> TEKFDFGTMVQWAYDHKYAEESKIAYEYALAAGSDSNARAFLATNSQAKHVKDCATMVRHYLRAETQALSMPAYIKARCKLATGEGSWKSILTFFNYQNIELITFINALKLWLKGIPKKNCLAFIGPPNTGKSMLCNSLIHFLGGSVLSFANHKSHFWLASLADTRAALVDDATHACWRYFDTYLRNALDGYPVSIDRKHKAAVQIKAPPLLVTSNID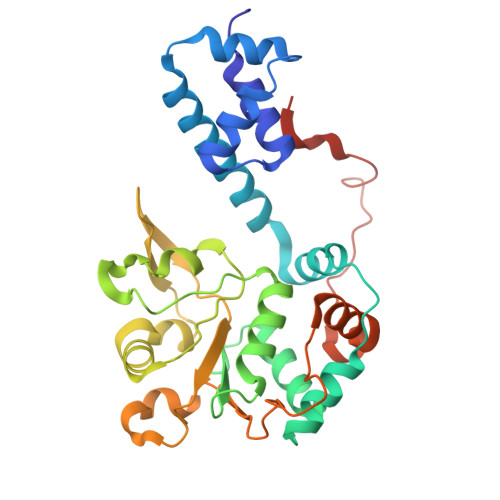VQAEDRYLYLHSRVQTFRFEQPCTDESGEQPFNITDADWKSFFVRLWGRLDLIDEEEDSEEDGDSMRTFTCSARNTNAVD>MPLPSPNLDDRRFQQFVDDAKRYIQQRAPEWTDHNVSDPGVTLVETVAHMADQIVYRLNRVPDKNHLAFLDLVGITLFPPSAARTDVTFWLSAPQEDAILVPVGTEVATLRTERDEAVVFATEQDLRIVPCTMGRLVTQVSGEAVSDRTTDLAESKDVLCFAEAPNPG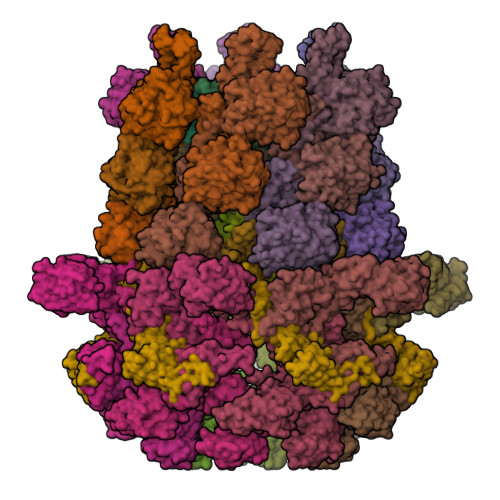DCMLIGLSAAVPDCALALELDSRVDGVGVDPRQPPLVWEAWTEDGWQSCEVDRDGTGGLNRPGDVVLHIPGGHVLSRNGGHEAGWIRCRVTEPLSGQPFYTTSPTIRSAEAYTIGGTTGSIHAETVLDEPLGESTGLPGQRLRLEHAPVVAGEPSVLLQTAADDGWQDWQVVPHFSGSHPDDHHITVDATTGEIAFGPAVREADGTLRQYGAVPPKGAVIRARRYRTGGGRAGNVARGAVQVLRTSIPYVSEVVNREAALGGVDGETIEEAKLRAPITLRAQERAVTLRDYEELARRAAPETARITCLEGAENEYGAHAVRVLVVPQAVPDPGGRLRFEQLVPGDALLNRITRHLDERRLIGTRLAVGPPYYQGVTVVATVHAFRDVDADRVRRQTHDALYRHLDPLTGGSDGKGWPFGRPVQTGELFAVLQRVPGVELVDEVVLHPADPLTGKRGDPTNRIDLDAPALVFSYDHRVRVIGDSA[12x];>MPSYLSPGVYVEEVASGSRPIEGVGTSVAAFVGLAPTGPLNEPTLVTNWTQYVAAFGDFTGGYYLAHSVYGFFNNGGSAAYVVRVGGSAEDAAADGSVNGAAAPAAVTGSTAKALPAAEPKQLGTFAVTATAAGQSGPLTVEVADPEGEGPAERFKLIVKDGDKPVETFDVSAKKGNRSYVVTQVKERSKLITVTEAAPSAQLVRPENQSLTLPAPPSAAPAVPAGQAESAHPGPAQYLGDSSDRTGFGGLEAIDEISMVAVPDLMAAYQRGAIDLEAVKAVQLGLIAHCELMGDRVAIIDPPPNQNARQIRVWRQETAGYDSKYAALYYPWIKSFDPATGQSRLVPPSGHVAGIWARNDSERGVHKAPANEVVRGAVDLELQITRGEQDLLNPIGVNCIRSFPGRGIRVWGARTLSSDPAWRYLNIRRYFNYLEESILIGTQWVVFEPNDHNLWARIRRNVSAFLVNEWRNGALFGQSPDQAYYVKCDEETNPPESVDLGRVVCEIGIAPVKPAEFVIFRLAQFSSGGGELDE[18x];>[6x]MKPASQRGSVDGLGSSLPIASMLPAVFADDDLALRFVAGLDDVLAPILNVLDCLDTYFDPALTPADFAQWLGTWVGAETDGTEAEPMLRAAVAAAARLHRVRGTLQGLSETVRLAFGVAPEITESGGATWNARPLGPFPGRPRPQLHVALRLPEPRPVDVHRLDALVAAARPAHMPYTVEVTASERTPER;>[6x]MAKSSKGAGKSLVRANLAIHEPPTGKSTSPGGLIKRFPFEFNPAQLSISQRSQWKATPTAAVRKAAKPQFMGAEPREMTLEIFLDSSMKPGGNTVMKKVESLLICCEVTAKSLAAKQPSPPWVIFEWGSFSTARFNAYVASIETQYTLFGTAGVPIRATCQMGLVEIPGPTPNQNPTSGALTAQRVHRVVAGDSLQSLAWSEYGSANAWRVIAEANGIDDPSHLPTGTELILPATEEVPH;>[6x]MAEQFVGSGWSFPLRIGPTGGIALVSGEQEVEEAMRLILATAPGERPMRPEFGCAIHDLVFAPVNEQTAGRIQHEVYVTLDRWEPRIEVHDVDVTTGEEQNVLFIDVRYSIRGTNNPRSLVFPFYVIPSHDEPDLPDAPAGLPGSPESDR;>[6x]MTRKDPGSSIWFSLAIDGESLGYFNGCEGLSTQVEVEQRQEGGNNGFVWQLPTRVTYSNIRLTRPLTPDTAKVAKWISSVQTGIQRPTAQISALRADGSLVARWGLIDVLPVSWQGPSLDPGSASVANEVLEIAHHGFTD;>MSLPKPEDVLVAPNFGIQIDGVMVEYLNSVSNLQIEQDVIRYQQNQGTTGRNNVTLMPGVAKDGSVQVERGMSQSSVFTQWINDSMAGRMATARKNATIIVMDYEDNPVKRWNLRNAWCSKVVAGTLKAGDTNALTETITIVFEELVVE[6x]>RSMEDENVKKFIKEFEDTKIMPVRKGTKTTRTEKFYLVFTEWVKLLQRVENNDVITTVFIKQLVEKGVISDTDNLLTFVKSSLELSVSSFKESDPTDEVFIAIDALGSLIIKLLILQDFKDDTRRDYINAIFSVIVLVFAKDHSQEGTTFNERPYFRLFSNILYEWATIRTHNFVRISD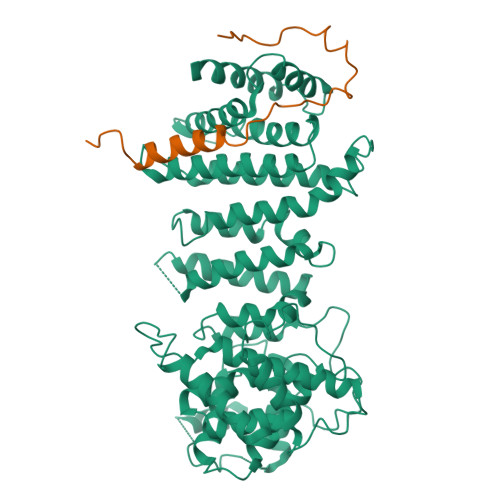SSTRQELIEFDSVFYNTFSGYLHALQPFAFPGFSFAWVTLLSHRMLLPIMLRLPNKIGWEKLMLLIIDLFKFLDQYTSKHAVSDAVSVVYKGTLRIILGISNDMPSFLIENHYELMNNLPPTYFQLKNVILSAIPKNMTVPNPYDVDLNMEDIPACKELPEVFFDPVIDLHSLKKPVDNYLRIPSNSLLRTILSAIYKDTYDIKKGVGYDFLSVDSKLIRAIVLHVGIEAGIEYKRTSSNAVFNTKSSYYTLLFNLIQNGSIEMKYQIILSIVEQLRYPNIHTYWFSFVLMNMFKSDEWNDQKLEVQEIILRNFLKRIIVNKPHTWGVSVFFTQLINNNDINLLDLPFVQSVPEIKLILQQLVKYSKKYTTSEQDDQ[6x];>GPDSMDPYDALGNAVDFLDARLHSLSNYQKRPISIKSNIIDEETYKKYPSLFSWDKIEASKKSDN[6x]>MADNIVLKTILQSEALQKYIFDTNVYPREHEQLKRIRDATFKKYGYRAELSVPPDEGLFLSMLLKLMNAKKTLEIGVFTGYSLLTTALALPHDGQIVAIDPNREAFEVGLPFIQKAGVEHKINFIESDAISVLNEMLSDEGKLKMEFDFVFVDADKPNYINYHEQAIKLVKVGGVIAYDNTLWYGSVVSNEEEVPERLRASQKPIIELNKYLASDPRIEITQISIGDGVTLCRRIL[2x]

Here, we identify two O-methyltransferases from tea plant: CsFAOMT1 that has a specific O-methyltransferase activity on the 3ʹʹ-position of EGCG to generate EGCG3′′Me, and CsFAOMT2 that predominantly catalyzes the formation of EGCG4″Me. To explain the specificity of CsFAOMT1 and CsFAOMT2, we crystallized both in the presence of EGCG and S-adenosyl-L-homocysteine (SAH), a by-product of the cofactor SAM and determined the structures at a resolution of 2.0 Å for CsFAOMT1 and 2.0 Å for CsFAOMT2. The electron densities for SAH and Mg2+ are unambiguously assigned, but EGCG was not found in either structure. The structural overlap of the monomers of CsFAOMT1 and CsFAOMT2 revealed a root mean square deviation of 0.36 Å over the Cα atom of 190 aligned residues, with the most striking difference occurring in an α-helix (α9) near the substrate binding pocket.

CsFAOMT1 exhibits significant 3″-O-methyltransferase activity to convert EGCG to EGCG3″Me in a Mg2+-dependent manner. In CsFAOMT1, this α-helix is bent toward the pocket, creating a deep and narrow cleft for substrate binding, whereas in CsFAOMT2 the corresponding α-helix is bent in the opposite direction, resulting in a relatively open and shallow pocket. To clarify the exact roles of these residues in substrate binding, we replaced SAH with SAM and then docked EGCG in the structure of CsFAOMT1. EGCG is embedded in a narrow and deep cleft formed by two α-helices, α3, and the bent α-helix α9, with both the A-ring and B-ring anchored through hydrogen bonds. Briefly, Y46 from α3 interacts with the 7-OH on the A-ring. For the B-ring, K156 and two residues from α9, R197 and S201, recognize 3′-, 4′- and 5′-OH, respectively. Notably, both CsFAOMT1-Y184 and CsFAOMT1-Y184R could form a hydrogen bond with the carbonyl group on the galloyl moiety, thereby positioning the D-ring into the active site, which may account for the specificity of CsFAOMTs to the D-ring of EGCG. The difference is that CsFAOMT1-Y184 helps to locate the 3″-hydroxyl on the D-ring close to the methyl group on SAM; substituting the tyrosine with an arginine that contains a longer side chain pushes the D-ring into a deeper pocket, resulting in the replacement of 3″-hydroxyl group by 4″-hydroxyl group close to the methyl group on SAM. Furthermore, we found a hydrophilic residue E49 in CsFAOMT1 that is in the proximity of the 5″-OH of EGCG and might be involved in the recognition of it through water-mediated hydrogen bonds, explaining why only EGCG3″Me was generated by CsFAOMT1. The exchange of a single residue in CsFAOMT1 (Y184) with the corresponding residue in CsFAOMT2 (R184) appears to be sufficient to confer apparent 4″-methyltransferase activity on CsFAOMT1, although the activity is much lower than that of CsFAOMT2.> MMQNLKKFMSKTIQVQPVSFNQIPKAFYNFPEYRTGGVQANPGITAKRIIKCIGERLRKYDPARWENVPITFKTHFR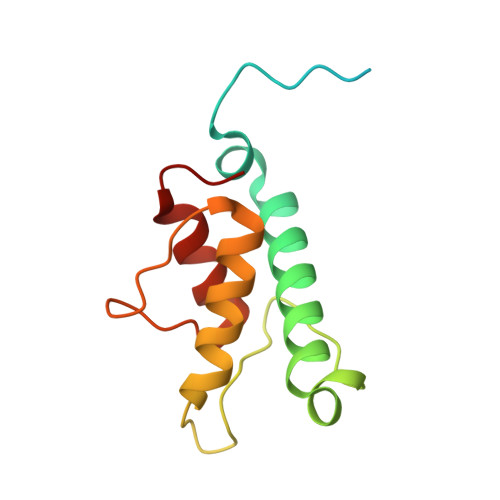DENGYSDVATSIQIHDALEREFGIDIKDRLALVTDVETAFYIVMSHHDPL5-[[4-[4-methyl-2-(methylamino)-1,3-thiazol-5-yl]pyrimidin-2-yl]amino]-~{N}-(3-morpholin-4-ylpropyl)-1~{H}-indole-2-carboxamide 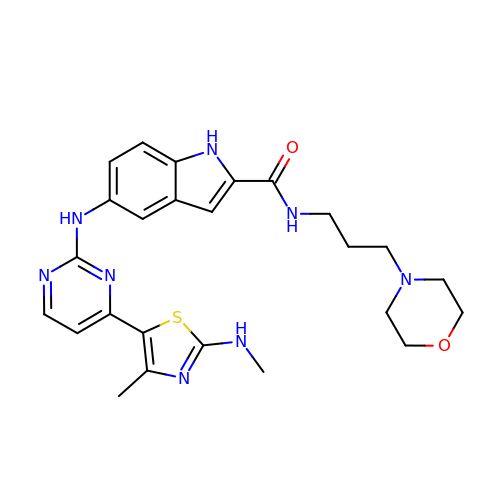| C25 H30 N8 O2 S | OTGQZMLMXDRMMX-UHFFFAOYSA-N SINAPOYL COENZYME A | C32 H44 N7 O20 P3 S | 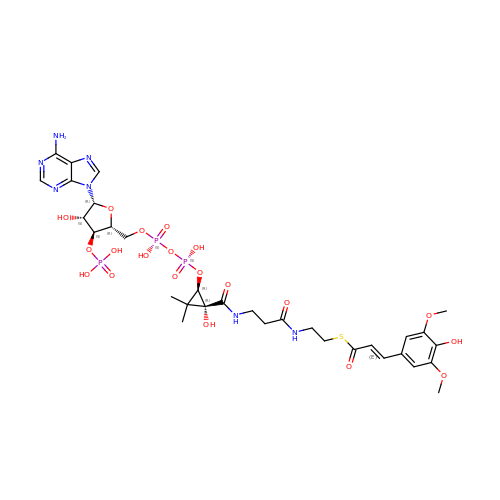HJGDVDUGXUSOGA-ADTMLPBESA-N(2S)-2-({2-deoxy-2-[(hydroxycarbamoyl)amino]-alpha-D-glucopyranosyl}oxy)butanedioic acid | C11 H18 N2 O11 | 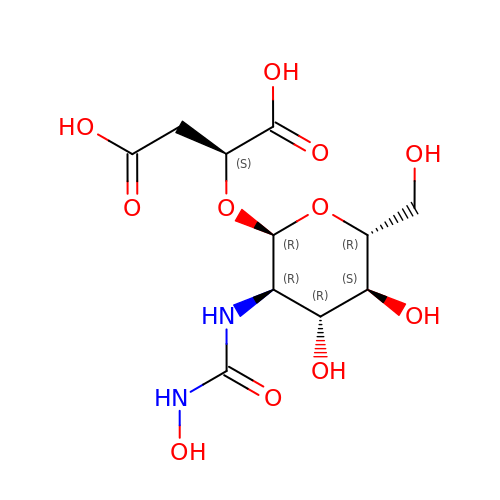QOPUTRBEPJZLTE-NKQVSKEESA-N CAFFEIC ACID | C9 H8 O4 | 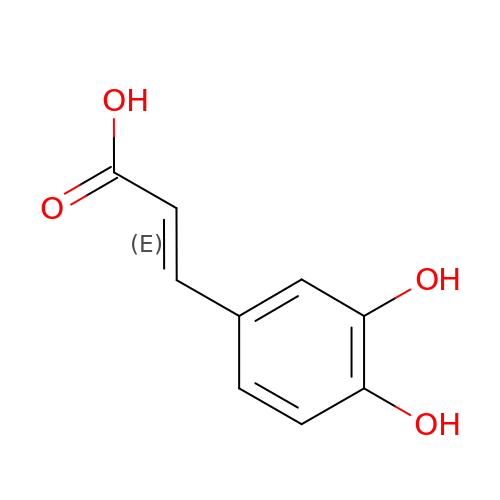QAIPRVGONGVQAS-DUXPYHPUSA-N>[2x]KIPNFVVPGKCASVDRNKLWAEQTPNRNSYAGVWYQFALTNNPYQLIEKCVRNEYSFDGKQFVIKSTGIAYDGNLLKRNGKLYPNPFGEP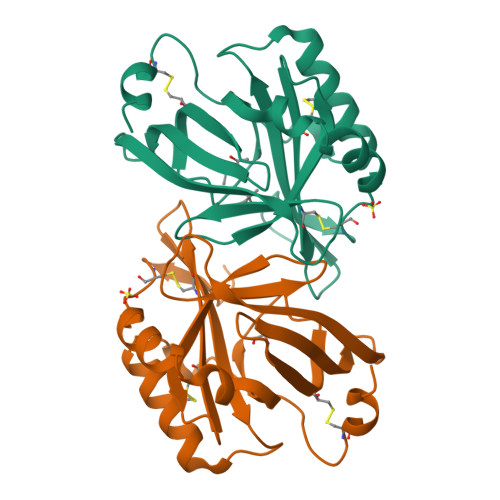HLSIDYENSFAAPLVILETDYSNYACLYSCIDYNFGYHSDFSFIFSRSANLADQYVKKCEAAFKNINVDTTRFVKTVQGSSCPYDTQKTV>[2x]AAVIEKRATCSNGKTVGDASCCAWFDVLDDIQQNLFH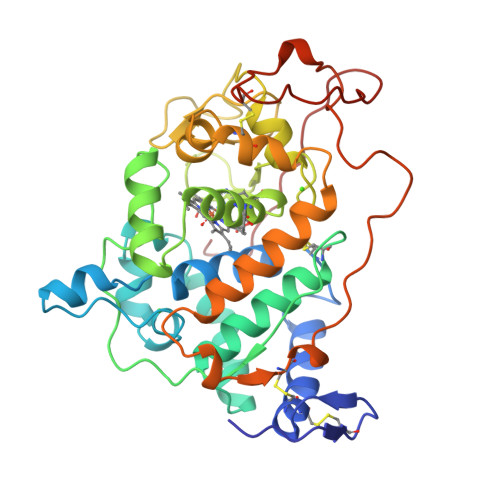GGQCGAEAHESIRLVFHDSIAISPAMEAQGKFGGGGADGSIMIFDDIETAFHPNIGLDEIVKLQKPFVQKHGVTPGDFIAFAGAVALSNCPGAPQMNFFTGRAPATQPAPDGLVPEPFHTVDQIINRVNDAGEFDELELVWMLSAHSVAAVNDVDPTVQGLPFDSTPGIFDSQFFVETQLRGTAFPGSGGNQGEVESPLPGEIRIQSDHTIARDSRTACEWQSFVNNQSKLVDDFQFIFLALTQLGQDPNAMTDCSDVIPQSKPIPGNLPFSFFPAGKTIKDVEQACAETPFPTLTTLPGPETSVQRIPPPPGA> SNAMNVWQVVGYKHSGKTTLMEKWVAAAVREGWRVGTVKHHGHGGEPARPEGVDSVRHERAGAVATAVEGDGLLQLHLRRPLWRLDDVLALYAPLRL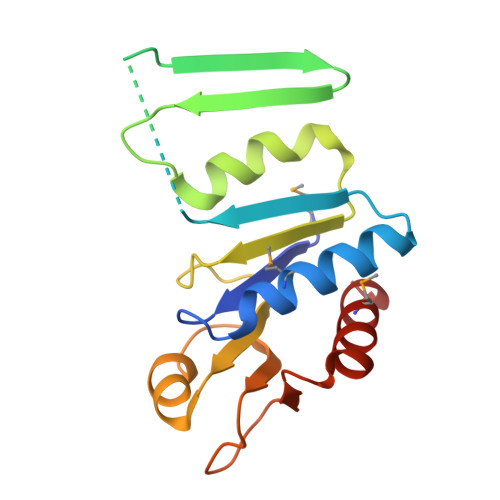DLVLVEGYKQERHPKVVLVRSEEDWASLQHLANIRAVIAWEPLEGPLAHPVFSLADDDEYIPWLMNEVRTRT> AEIYNKDGNKVD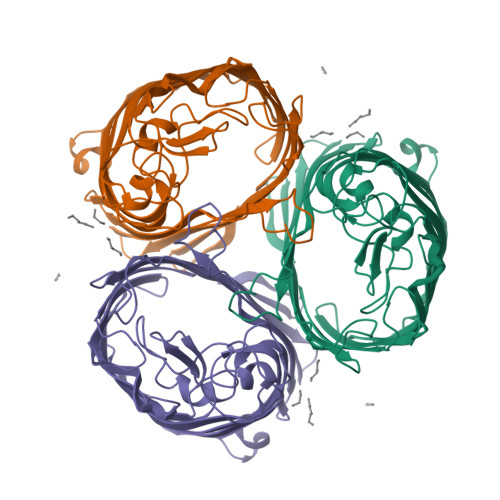LYGKAVGLHYFSKGNGENSYGGNGDMTYARLGFKGETQINSDLTGYGQWEYNFQGNNSEGADAQTGNKTRLAFAGLKYADVGSFDYGRNYGVVFDALGYTDMLPEFGGDTAYSDDFFVGRVGGVATYRNSNFFGLVDGLNFAVQYLGKNERDTARRSNGDGVGGSISYEYEGFGIVGAYGAADRTNLQEAQPLGNGKKAEQWATGLKYDANNIYLAANYGETRNATPITNKFTNTSGFANKTQDVLLVAQYQFDFGLRPSIAYTKSKAKDVEGIGDVDLVNYFEVGATYYFNKNMSTYVDYIINQIDSDNKLGVGSDDTVAVGIVYQF> MKKLFLVFWWHMHQPLYREPYTGEYLLPWTFFHAVKDYYDMPAYLKDFEIKLNFNLTPVLIDQIQEYAQGKAKDVFLEAIRKDPDDLEKEEVEKLIEFTKLNYEKPIYRFERIRELMNKEKLNREELLDLQTLNLLAWCGRTLRKDLKDLLNKGRNYTQEEKEYVLNKYFEIIKKTLSIYREIKEEGKGSVSTSPYYHPLIPILLNPNCVYETTPNVKIPDFAVSFREDASKHVELAKEKYFEIFGEHPVYMWPPEASVSNEALELYYEKGINMLATDEVILKNSVERASPYLRYYFRELISVFFRDKTLSDLI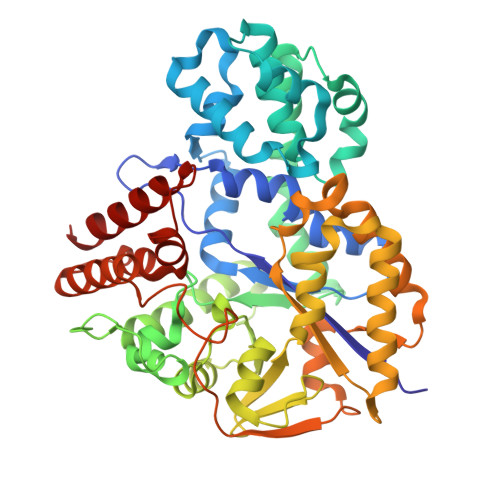GFSYHAWNAEDAVRDFIGRLKKIHESVDFQPVVFVVLDGENCWEYYEENGIPFLEKLYSTLEKEEWIETLTLEEAMRKEDVKTEVIESVKAGTWFDGNFLKWIGNKEKNEYWKILIEAKKKAKNDYILVAEGSDWFWWQGEEKAPFVEVFDKLFRSFVRRAQE>MVTFHTNHGDIVIKTFDDKAPETVKNFXDYCRE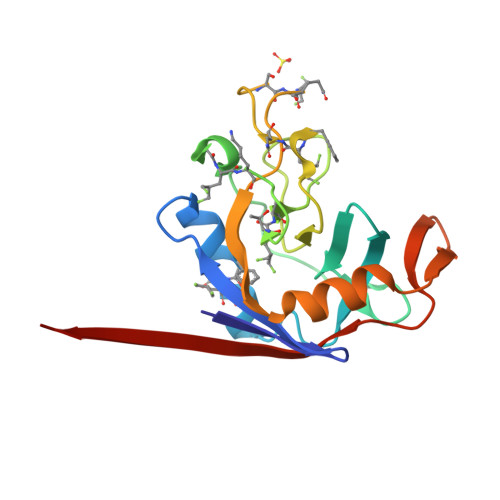GFYNNTIFHRVINGFMIQGGGFEPGMKQKATKEPIKNEANNGXKNTRGTXAMARTQAPHSATAQFFINVVDNDFXNFSGESXQGWGYCVFAEVVDGMDVVDKIKGVATGRSGMHQDVPKEDVIIESVTVSEHHHHHH[4x]> GUGUGCCCGGCAUGGGUGCAGUCUAUAGGGUGAGAGUCCCGAACUGUGAAGGCAGAAGUAACAGUUAGCCUAACGCAACUGCGCCGUGGCGACAUGGCGUGGGAAGGAAGCGGACGGCAAACCUUCGGUCUGAGGAACACGAACUUCAUAUGAGGCUAGGUAUCAAUGGAUGAGUUUGCAUAACAAAACAAAGUCCUUUCUGCCAAAGUUGGUACAGAGUAAAUG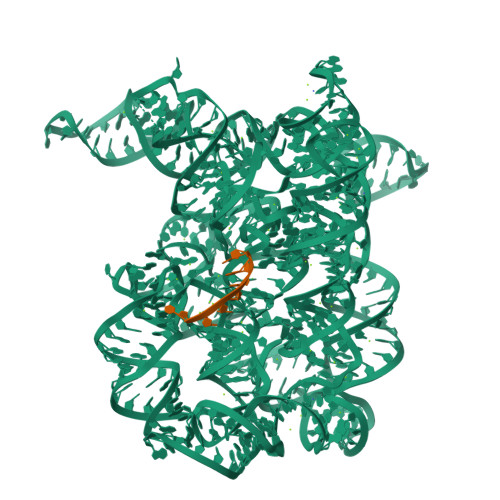AAGCAGAUUGAUGAAGGGAAAGACUGCAUUCUUACCCGGGGAGGUCUGGAAACAGAAGUCAGCAGAAGUCAUAGUACCCUGUUCGCAGGGGAAGGACGGAACAAGUAUGGCGUUCGCGCCUAAGCUUGAACCGCCGUAUACCGAACGGUACGUACGGUGGUGUGGCAGGGGCGCUUCGGCCCCCUAUGCCGAU;> CUGUUAX> TKDQRDVNVFKKVLENIGNAVTQFNNDILAYTGGDANHLIHDGDAIIKATENGLQELGPQPPLSLTEALALV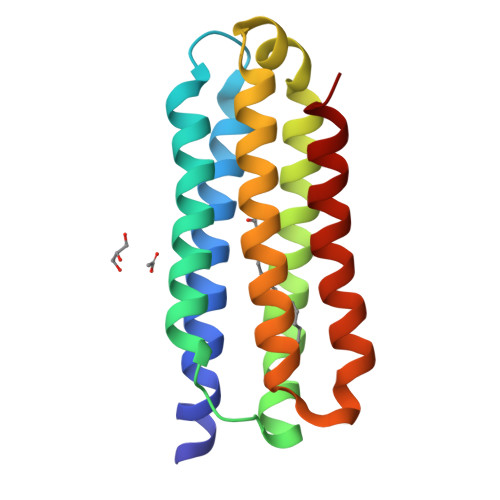GPVQGVNKLIMKTVDHLIEKKGPLVGGGYGPQVKASLQKQAHAAVTLSELVSSKVPSPLAPISKQLSDQVAQALQKGIEAFSI> SNAASGSALIFDEEMSRYKLLWTDPACEIEVPERLTVSYEALRTHGLAQRCKAVPVRQATEQEILLAHSEEYLEAVKQTPGMNVEELMAFSKKYNDVYFHQNIYHCAKLAAGATLQLVDSVMKREVRNGMALVRPPGHHSQRSAANGFCVFNNVAFAALYAKKNYNLNRILIVDWDVHHGQGIQYCFEEDPSVLYFSWHRYEHQSFWPNLPESDYSSVGKGKGSGFNINLPWNKVGMTNSDYLAAFFHVLLPVAYEFDPELVIVSAGFDSAIGDPEGEMCALPEIFAHLTHLLMPLAAGKMCVVLEGGFNLTSLGQSVCQTVHSLLGDPTPRISGLGTACDSALESIQNVRNVQSSYWSSFKHLAQSETNPKRPRLDATNGGPKESSEPASESNPKKTAQDIVWPEPLKRMPASVRTVVVPPPGVELTLPKNCQHSGDISESTAKEVQRIRDKHFHDLTDQNILRSLGNIISVLDRMMRSDEVCNGCVVVSDLSVSVQCALQHALTEPAERVLVVYVGDGELPVKTNDGKVFLVQICTKETEDKCVNRLTLCLREGESLTAGFMQALLGLILPVAYEFNPALVLGIVEETAAKTRLMRVWGHMTC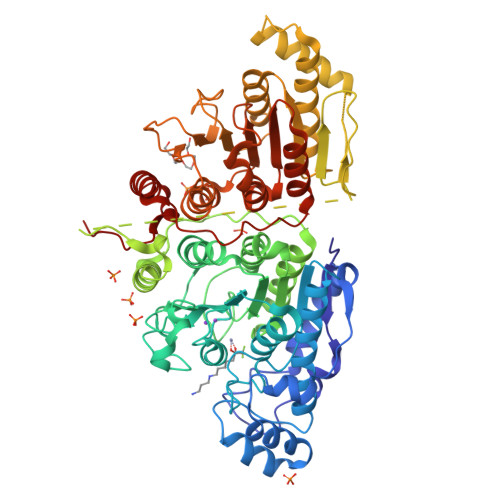LIQGLARGRMLTLLQGYDKDLLELTVSALSGASISPLGPLRAPKPEDVEMMEKQRQRLQERWGLLRCTVSESW>[4x]SNAENSEVIKDLYEYL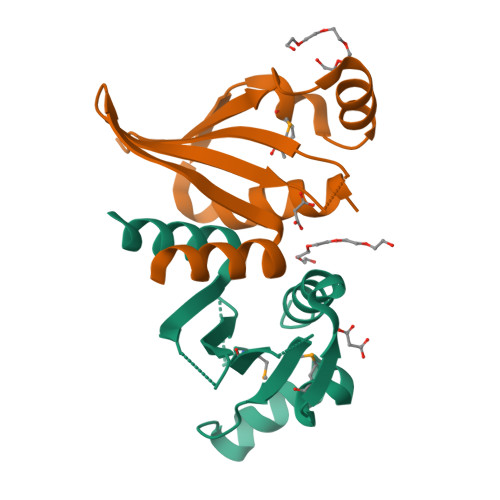CNVRVHKSYEDDSGLWFDISQGTHSGGSSDDYSIMDYKLGFVKGQAQVTEVIYAPVLKQRSTEELYSLQSKLPEYMFETLSFPLSSLNQFYNKIAKSLNK VhCBP is a periplasmic chitooligosaccharide-binding protein mainly responsible for translocation of the chitooligosaccharide (GlcNAc)2 across the double membranes of marine bacteria. The chitooligosaccharide-specific SBP is localized to the periplasmic compartment of the bacterial cell wall and serves as a mobile component of the (GlcNAc)2-specific ABC transporter. SBPs share a common structural feature comprising two domains connected by a flexible hinge region. VcCBP and VhCBP belong to cluster C/subcluster IV (C-IV), members of which are specific for oligosaccharides, including mannooligosaccharides, cellooligosaccharides, and chitooligosaccharides.

The F411A mutation did not affect the hydrogen bonds but eliminated the hydrophobic interaction with the N-acetyl methyl group of the reducing-end GlcNAc. Mutation of Phe411 lowered the favorable contribution of the enthalpy change, suggesting a role of Phe411 in masking the N-acetyl group from water molecules, avoiding direct contact with water and forming a hydrophobic interaction with the N-acetyl methyl group. The effects on ΔG° in the other mutants (E10A, N204A, S221A, N409A, and F411A) were moderate, although one mutation had been introduced into an amino acid with a high degree of conservation (Asn204).

> AERSELTIHPKEFTTFVRNFNPFLGATNLHTTTDFIYEPLVVFNEMHGNTPVFRLAENFQMSDDLMSVTFDIRKGVKWSDGEAFTADDVVYSFNLVKEKPELDQSGINSWVTGVEKVNDYQVKFRLSEANSNVPYEIAKVPVVPKHVWSKVKDPSTFTNENPVGSGPFTVIDTFTPQLYIQCENPNYWDAANLDVDCLRVPQIANNDQFLGKVVNGEMDWTSSFVPDIDRTYAAASPKHHYWYPPAGTQAFVVNFKNPDAAKNEALTNVDFRRAFSMALDRQTIIDIAFYGGGTVNDFASGLGYAFEAWSDEKTHDKFKAYNSYNAEGAKKLLAKAGFKDVNKDGFVDTPSGKSFELLIQSPNGWTDFNNTVQLAVEQLAEVGIKARARTPDFSVYNQAMLEGTYDVAYTNYAHGADPYTYWNSAYNSALQSGDGMPRFAMHFYKNEKLDGLLNSFYKTADKQEQLEIAHGIQQIIAQDQVTIPVLSGAYMYQYNTTRFTGWWNEENPKGRPNIWAGIPERLLHVLDLKPVKHHHHHH2-amino-4-oxo-1,4-dihydropteridine-7-carboxylic acid | C7 H5 N5 O3 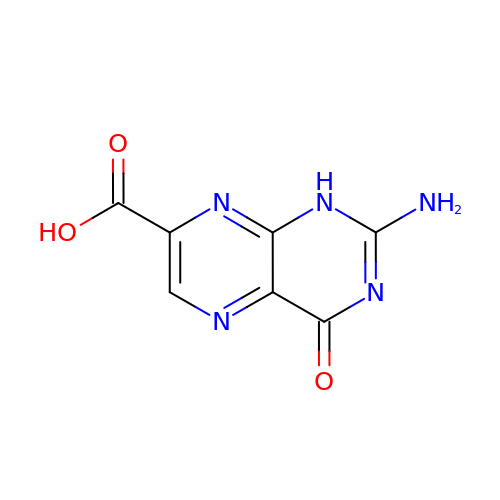| NZLJLZVXWBEGCE-UHFFFAOYSA-N>GSDPIKISIPRYVLCGQGKDAHFEFEVKITVLDETWTVFRRYSRFREMHKTLKLKYAELAALEFPPKKLFGNKDERV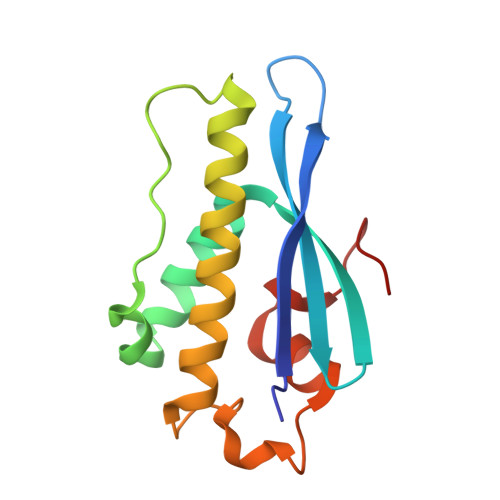IAERRSHLEKYLRDFFSVMLQSATSPLHINKVGLTLSKHTICEFSPFFKKGVFDYS[3x]>GSEQKKRRLEEGTRANSVAESSPPFPLRSKTSVGSTNSQITETKNKQGVYPITESNLRILEGEDRSEKAKELLKKYVSNVFENEKTLYIYCKYVMLHYGKDLVNPNEVDSLEFQIINGGITNILIKVKDMSKQAKYLIRLYGPKTDEIINREREKKISCILYNKNIAKKIYVFFTNGRIEEFMDGYALSREDIKNPKFQKLIAKNLKLLHDIKLNENLYKELQVTQKVPGTRPSFLWNTIWKYFHLLNEERKKICSFDAKANILKLIDFDVLRDSIVEVESLCKRENSPIVLCHCDLLSSNIIN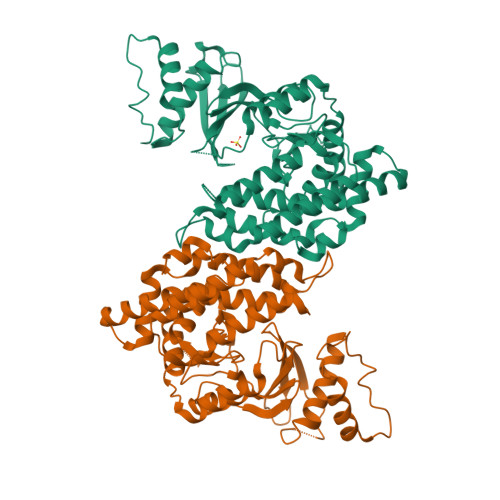TVGGGEAGELGEAGETGEGGETGEGGETGEGGETGEGGEGDSISFIDFEYSCPMERAYDIANHFNEYAGFNCDWDLTPSKEEEYHFIMHYLGTDDEELINQLIREIQPFYICSHINWGLWSLLQGMHSSIDFDFINYGMTRLTASCLPIFRSKV[4x]> EQARPADDALAALGAQLFVDPALSRNATQSCATCHDPARAFTDPREGKAGLAVSVGDDGQSHGDRNTPTLGYAALVPAFHRDANGKYKGGQFWDGRADDLKQQAGQPMLNPVEMAMPDRAAVAARLRDDPAYRTGFEALFGKGVLDDPERAFDAAAEALAAYQATGEFSPFDSKYDRVMRGEEKFTPLEEFGYTVFITWNCRLCHMQRKQGVAERETFTNFEYHNIGLPVNETAREASGLGADHVDHGLLARPGIEDPAQSGRFKVPSLRNVAVTGPYMHNGVFTDLRTAILFYNKYT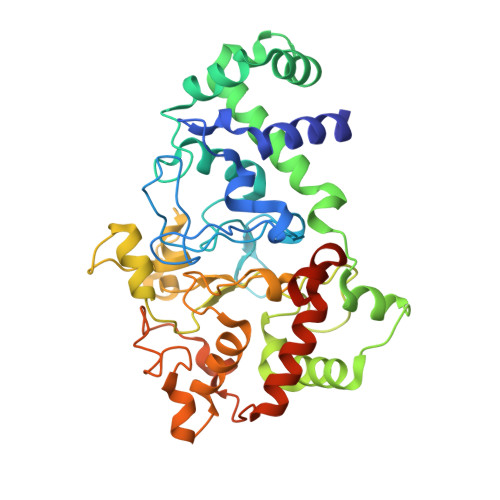SRRPEAKINPETGAPWGEPEVARNLSLAELQSGLMLDDGRVDALVAFLETLTDRRYEPLLEESRAAQKDHHHHHH>MGNNRVVYLKYAKAEDLVEVLKGVSENLQAEKGTGQPTTSKRNEVMIAAHADTNSLVLTAPQDIMNAMLEVIGQLDIRRAQVLIEALIVEMAEGDGINLGVQWGSLESGSVIQYGNTGASIGNVMIGLEEAKDTTQTKAVYDTNNNFLRNETTTTKGDYTKLASALSSIQGAAVSIAMGDWTALINAVSNDSSSNILSSPSITVMDNGEASFIVGEEVPVITGSTAGSNNDNPFQTVDRKEVGI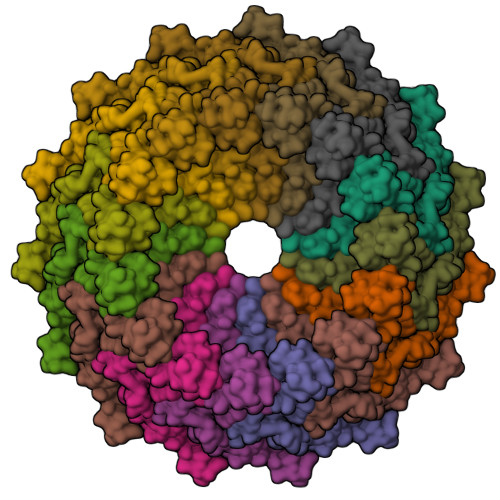KLKVVPQINEGNSVQLNIEQEVSNVLGANGAVDVRFAKRQLNTSVMVQDGQMLVLGGLIDERALESESKVPLLGDIPLLGQLFRSTSSQVEKKNLMVFIKPTIIRDGVTADGITQRKYNYIRAEQLFRAEKGLRLLDDASVPVLPKFGDDRRHSPEIQAFIEQMEAKQWSHPQFEK[15x]>[2x]RPGLPVEYLQVPSASMGRDIKVQFQGGGPHAVYLLDGLRAQDDYNGWDINTPAFEEYYQSGLSVIMPVGGQSSFYTDWYQPSQSNGQNYTYKWETFLTREMPAWLQANKGVSPTGNAAVGLSMSGGSALILAAYYPQQFPYAASLSGFLNPSESWWPTLIGLAMNDSGGYNANSMWGPSSDPAWKRNDPMVQIPRLVANNTRIWVYCGNGTPSDLGGDNIPAKFLEGLTLRTNQTFR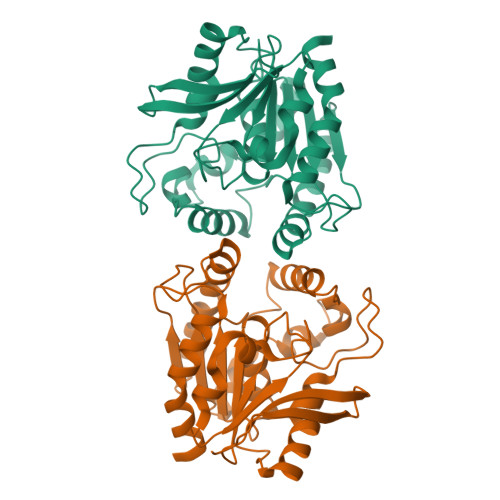DTYAADGGRNGVFNFPPNGTHSWPYWNEQLVAMKADIQHVLNG VanR is the response regulator of the VanR–VanS two-component system, which controls the expression of a vancomycin-resistant phenotype in many bacteria, including soil microbes such as Streptomyces coelicolor as well as serious human pathogens such as vancomycin-resistant enterococci (VRE; Hong et al., 2008). VanR is composed of an N-terminal receiver domain, which contains the conserved aspartate that is the target for phosphorylation, and a C-terminal DNA-binding domain, which enables VanR to function as a transcription factor. Upon phosphorylation, VanR is thought to dimerize, bind to promoters within the vancomycin-resistance operon, and activate transcription of the resistance genes. VanR belongs to the OmpR/PhoB class of response regulators.

X-ray crystal structures were determined for the inactive and activated states at resolutions of 2.3 and 2.0 Å, respectively. Both activity states crystallized in the same P6522 space group but with different unit-cell dimensions; in both crystal forms the asymmetric unit contained a monomer. For both conformational states, no electron density was observed for the 12 C-terminal residues (221–232), suggesting a highly flexible C-terminal tail. While one might expect long linkers such as those in the VanRSc structures to be highly flexible, the linkers are well ordered in the crystals of both activity states. In the structure of inactive VanRSc the linkers from two adjacent molecules in the crystal lattice associate in an antiparallel manner, leading to the formation of a symmetric pair of hydrogen bonds between the carbonyl O atom of Arg123 and the amide proton of Arg123′ of the symmetry mate, along with a similarly symmetric pair of hydrogen bonds between the side chain of Arg123 and the carbonyl O atom of Pro124′. In contrast, in the crystals of the inactive form of VanRSc none of the lattice contacts appear to correspond to biologically meaningful interfaces. The main structural differences between the two activity states center around the stability of α4 and the oligomeric state of the protein. Comparison of the two structures illustrates that phosphorylation of VanR is accompanied by a disorder-to-order transition of helix 4, which lies within the receiver domain of the protein. The inactive conformation of the protein does not appear intrinsically unable to bind DNA; rather, it is proposed that in the activated form DNA binding is enhanced by an avidity effect contributed by the receiver-domain dimerization.

> GMRVLIVEDEPYLAEAIRDGLRLEAIAADIAGDGDTALELLSVNAYDIAVLDRDIPGPSGDEIAERIVASGSGMPILMLTAADRLDDKASGFGLGADDYLTKPFELQELALRLRALDRRRAHSRPPVREIAGLRLDPFRREVYRGGRYVALTRKQFAVLEVLVAAEGGVVSAEELLERAWDENADPFTNAVRITVSALRKRLGEPGIIATVPGVGYRIDTAPVSEQAGGDGG> CG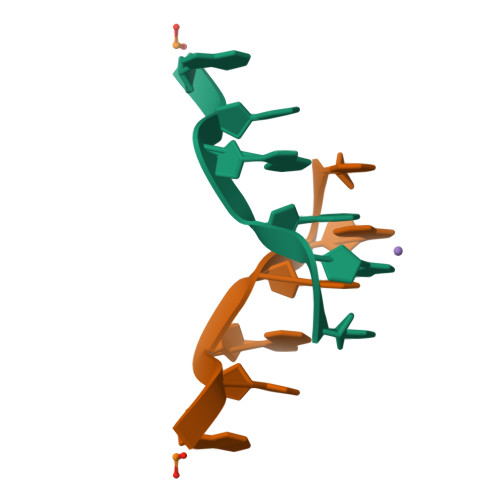TGCG> MAVKVEYDLKRLRNIGIAAHIDAGKTTTTERILYYTGRIHKIGEVHEGAATMDFMEQERERGITITAAVTTCFWKDHRINIIDTPGHVDFTIEVERSMRVLDGAIVVFDSSQGVEPQSETVWRQAEKYKVPRIAFANKMDKTGADLWLVIRTMQERLGARPVVMQLPIGREDTFSGIIDVLRMKAYTYGNDLGTDIREIPIPEEYLDQAREYHEKLVEVAADFDENIMLKYLEGEEPTEEELVAAIRKGTIDLKITPVFLGSALKNKGVQLLLDAVVDYLPSPLDIPPIKGTTPEGEVVEIHPDPNGPLAALAFKIMADPYVGRLTFIRVYSGTLTSGSYVYNTTKGRKERVARLLRMHANHREEVEELKAGDLGAVVGLKETITGDTLVGEDAPRVILESIEVPEPVIDVAIEPKTKADQEKLSQALARLAEEDPTFRVSTHPETGQTII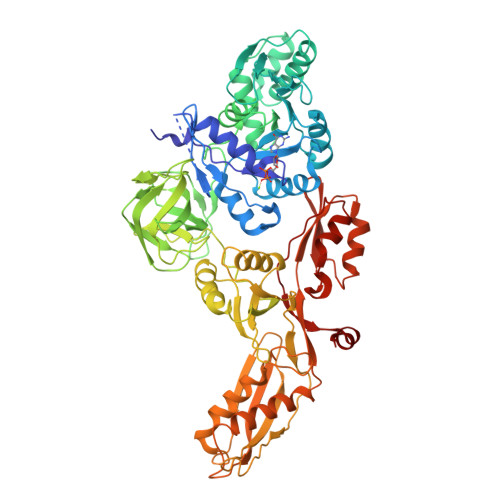SGMGELHLEIIVDRLKREFKVDANVGKPQVAYRETITKPVDVEGKFIRQTGGRGQYGHVKIKVEPLPRGSGFEFVNAIVGGVIPKEYIPAVQKGIEEAMQSGPLIGFPVVDIKVTLYDGSYHEVDSSAMAFKIAGSMAIKEAVQKGDPVILEPIMRVEVTTPEEYMGDVIGDLNARRGQILGMEPRGNAQVIRAFVPLAEMFGYATDLRSKTQGRGSFVMFFDHYQEVPKQVQEKLIKGQ> MLYGSSISAESMKVIAESIGVGSLSDDAAKELAEDVS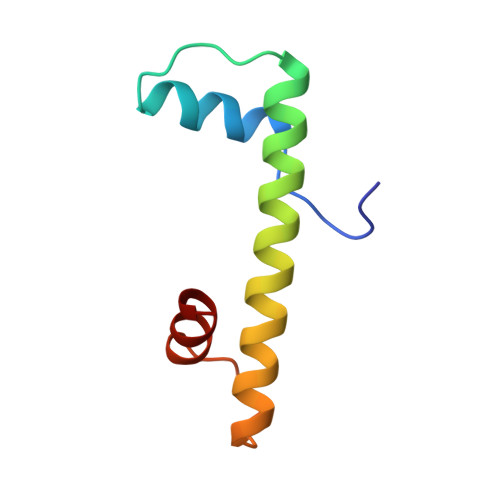IKLKRIVQDAAKFMNHAKRQKLSVRDIDMSLKV>[2x]AVSFIGSTENDVGP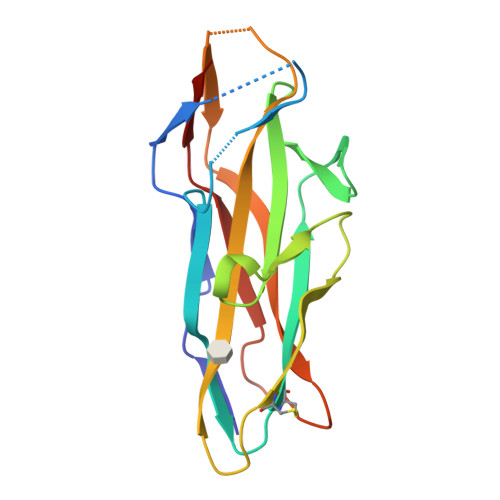SLGSYSRTHAMDNLPFVYDTRNKIGYQNANVWHISKGFCVGLDGKVDLPVVGSLDGQSIYGLTEEVGLLIWMGDTKYSRGTAMSGNSWENVFSGWCVGANTASTQGLSVRVTPVILKRNSSARYSVQKTSIGSIRMRPYNGSSAGSVQTTVNFSLNPFTLNDT CYTOSINE ARABINOSE-5'-PHOSPHATE | C9 H14 N3 O8 P | 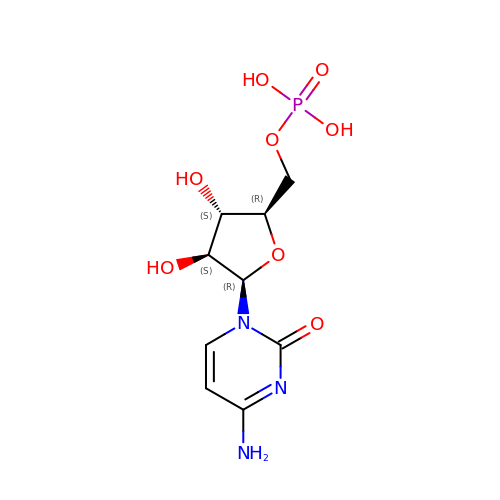IERHLVCPSMICTF-CCXZUQQUSA-N> MEH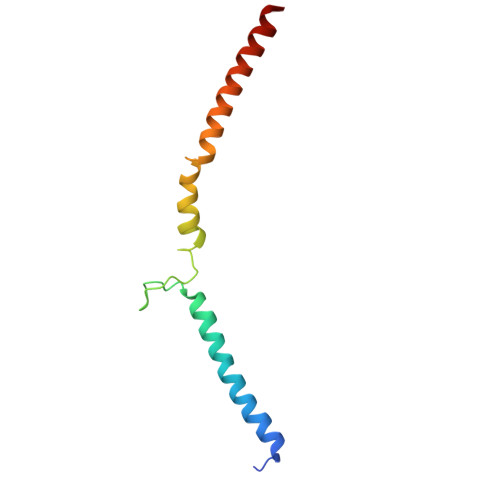NLSPLQQEVLDKYKQLSLDLKALDETIKELNYSQHRQQHSQQETVSPDEILQEMRDIEVKIGLVGTLLKGSVYSLILQRKQEQESLGSNSK> MAVTNEEIKTASKIVRRVSNVEAFDKSGSVFKGYQIWTDISPTIENDPNIMFVKCVVQQGSKKEKLTVVQIDPPGTGTPYDIDPTHAWNCNSQVDPMSFGDIGLLNHTNIPCVLDFLKHRYLKNQIYTTAVPLIVAINPYKDLGNTTNEWIRRYRDTADHTKLPPHVFTCAREALSNLHGVNKSQTIIVSGESGAGKTEATKQIMRYFASSKSGNMDLRIQTAIMAANPVLEAFGNAKTIRNNNSSRFGRFMQLVISHEGGIRYGSVVAFLLEKSRIITQDDNERSYHIFYQFLKGANSTMKSKFGLKGVTEYKLLNPNSTEVSGVDDVKDFEEVIESLKNMELSESDIEVIFSIVAGILTLGNVRLIEKQEAGLSDAAAIMDEDMGVFNKACELMYLDPELIKREILIKVTVAGGTKIEGRWNKNDAEVLKSSLCKAMYEKLFLWIIRHLNSRIEPEGGFKTFMGMLDIFGFEVFKNNSLEQLFINITNEMLQKNFVDIVFERESKLYKDEGISTAELKYTSNKEVINVLCEKGKSVLSYLEDQCLAPGGTDEKFVSSCATNLKENNKFTPAKVASNKNFIIQHTIGPIQYCAES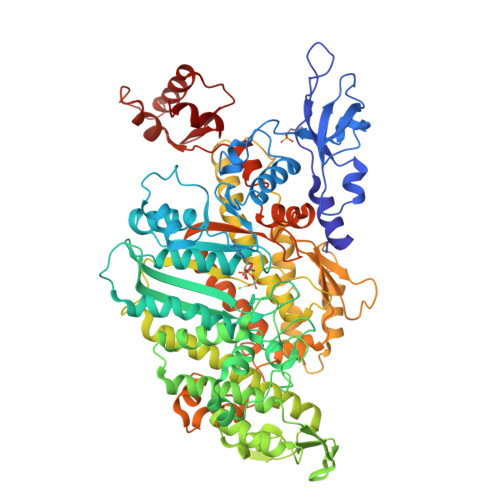FLLKNKDVLRGDLVEVIKDSPNPIVQQLFEGQVIEKGKIAKGSLIGSQFLNQLTSLMNLINSTEPHFIRCIKPNENKKPLEWCEPKILIQLHALSILEALVLRQLGYSYRRTFEEFLYQYKFVDIAAAEDSSVENQNKCVNILKLSGLSESMYKIGKSMVFLKQEGAKILTK> SLSNKLTLDKLDVKGKRVVMRVDFNVPMKNNQITNNQRIKAAVPSIKFCLDNGAKSVVLMSHLGRPDGVPMPDKYSLEPVAVELKSLLGKDVLFLKDCVGPEVEKACANPAAGSVILLENLRFHVEEEGKGKDASGNKVKAEPAKIEAFRASLSKLGDVYVNDAFDTAHRAHSSMVGVNLPQKAGGFLMKKELNYFAKALESPERPFLAILGGAKVADKIQLINNMLDKVNEMIIGGGMAFTFLKVLNNMEIGTSLFDEEGAKIVKDLMSKAEKNGVKITLPVDFVTADKFDENAKTGQATVASGIPAGWMGLDCGPESSKKYAEAVTRAKQIVWNGPVGVFEWEAFARGTKALMDEVVKATSRGCITIIGGGDTATCCAKWNTEDKVSHVSTGGGASLELLEGKVLPGVDALSNI

Phosphoglycerate kinase 1 (PGK1) is an ubiquitous enzyme expressed in all somatic cells that plays a central role in glycolysis where it provides energy in form of ATP through the reversible phosphotransfer reaction from 1,3-bisphosphoglycerate (1,3-BPG) to MgADP in order to produce 3-phosphoglycerate (3-PG) and MgATP in the presence of free magnesium. PGK1 is a monomeric enzyme of 417 amino acids formed by two distinct α-helical domains of equal size, the N- and C-terminal domains connected by a hinge region. The N-terminal domain binds 3-PG or 1,3-BPG while the C-terminal domain binds MgADP or MgATP. Two different crystallographic conformations of PGK1 have been already identified: the partially closed conformation, able to bind substrates, and the closed conformation, the catalytically competent state.

G166 is located in the 3-PG binding pocket interacting with the substrate C2 through its main carboxylic group. G166 is one of the residues lining the 3-PG binding site and its substitution for the bulky and negatively charged aspartate modifies the shape and the charge of the substrate binding pocket. The structure of G166D reveals that the aspartate Oδ is engaged in a salt bridge with the R38 NH1 (OD-(D166)-NH1(Arg38) = 3.3 Å) altering its capability of interacting with 3-PG. These modifications of the pocket impair the binding of 3-PG, that is not present in the structure, and the stabilization of the transition state through R38, thus affecting both kcat (5.9 s-1) with a 15-fold decrease, and KM (1.54 mM) increased 4- fold. Mutation of the other residues involved in 3-PG binding, R65W, a positively charged arginine with the non polar tryptophan, and G166D, a substitution of glycine with a negatively charged residue, leads to an increase in Km values and, in the case of G166D, also to a reduced turnover number. As shown in the structure, the introduction of a negatively charged residue in the 3-PG binding site alters the affinity of the protein for the substrate (which is not found in the structure) by occupying part of the binding site and by engaging the R38 in a new salt bridge. The occurrence of undetectable unfolding intermediates may be the case of R38M and G166D, as suggested by the non coincidence of the [Urea]0.5 values obtained by far-UV CD and fluorescence changes, mainly due to the differences in m value.>MAYSQGGGKKKVCYYYDGDIGNYYYGQGHPMKPHRIRMTHNLLLNYGLYRKMEIYRPHKATAEEMTKYHSDEYIKFLRSIRPDNMSEYSKQMQRFNVGEDCPVFDGLFEFCQLSTGGSVAGAVKLNRQQTDMAVNWAGGLHHAKKSEASGFCYVNDIVLAILELLKYHQRVLYIDIDIHHGDGVEEAFYTTDRVMTVSFHKYGEYYFPGTGDLRDIGAGKGKYYAVNFPMRDGIDDESYGQIFKPIISKVMEMYQPSAVVLQCGADSLSGDRLGCFNLTVKGHAKCVEVVKTFNLPLLMLGGGGYTIR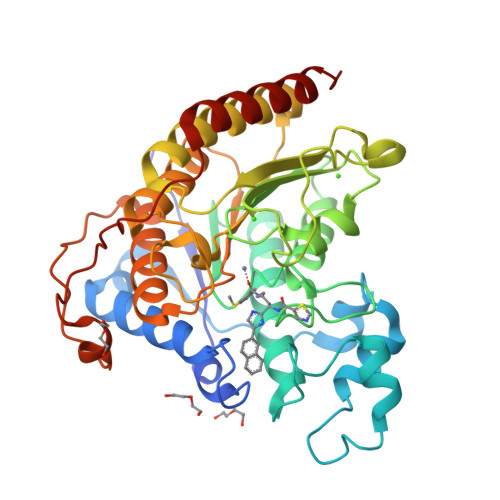NVARCWTYETAVALDCEIPNELPYNDYFEYFGPDFKLHISPSNMTNQNTPEYMEKIKQRLFENLRMLPH[3x]In P. aeruginosa, the gene PA0745 encodes a putative crotonase, named dspI, which has been shown to be responsible for the CDA biosynthesis. The structural studies confirmed the catalytic features of DspI as an enoyl-coenzyme A (CoA) hydratase that catalyzes the dehydration of 3-hydroxydecanoyl-CoA during CDA synthesis. DspI is a α/β protein composed of six perpendicular antiparallel β-strands surrounded by eleven α-helices. It can be divided into two domains: the N-terminal spiral domain (α1–α8 and β1–β6) and the C-terminal trimerization domain (α9-end).

The proteins were crystallized in two different space groups. The P31 form has six molecules and the P6322 form has only one molecule per asymmetric units. The atomic coordinates from the two space groups were refined at a resolution of 2.10 Å and 2.25 Å. In both crystal forms, the first eight residues have not been modeled because of the poor density in this region. The C-terminal segment (residue 252–272) is further missing in the P6322 form. Hexamer organizations could be generated by applying the symmetry operations in both crystal forms. The hexamer is a dimer of two stacked trimers and each subunit possesses the canonical crotonase fold. Although the crystal soaking and co-crystallization did not generate the substrate (or analogue) that bound the DspI structure, the 2Fo-Fc difference map around the active site in the P6322 form allowed us to model an acetic acid molecule in it. The hydroxyl group from the acetic acid points toward residue Glu126 and Glu146, implicating the possible binding pattern for the 3′ hydroxyl group of the CDA-CoA precursor 3-hydroxydecanoyl-CoA.

> MNTAVEPYKASSFDDTHKLTVEKHGHTALITINHPPANTWDRDSLIGLRQLIEHLNRDDDIYALVVTGQGPKFFSAGADLNMFADGDKARAREMARRFGEAFEALRDFRGVSIAAINGYAMGGGLECALACDIRIAERQAQMALPEAAVGLLPCAGGTQALPWLVGEGWAKRMILCNERVDAETALRIGLVEQVVDSGEARGAALLLAAKVARQSPVAIRTIKPLIQGARERAPNTWLPEERERFVDLFDAQDTREGVNAFLEKRDPKWRNCLEHHHHHH> CRLYYAGEFHKMREVILDSSEEDFIRSLSHSSPWQARGGKSGAAFYATEDDRFILKQMPRLEVQSFLDFAPHYFNYITNAVQQKRPTALAKILGVYRIGYKNSQNNTEKKLDLLVMENLFYGRKMAQVFDLKGSLRNRNVKTDTGKESCDVVLLD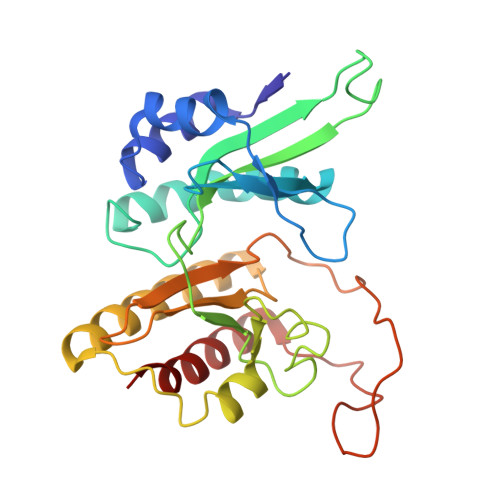ENLLKMVRDNPLYIRSHSKAVLRTSIHSDSHFLSSHLIIDYSLLVGRDDTSNELVVGIIDYIRTFTWDKKLEMVVKSTGILGGQGKMPTVVSPELYRTRFCEAMDKYFL> SNASIFKDLEALSFQSNASRNQDVFPILDLQELVICLQSCDFALATQENISRPTSDYMVTLYKQIIENFMGISVESLLNSSNQETGDGHLQEENENIYLDTLNVLVLNKICFKFFENIGVQDFNMTDLYKPEAQRTQRLLSAVVNYARFREERMFDCNS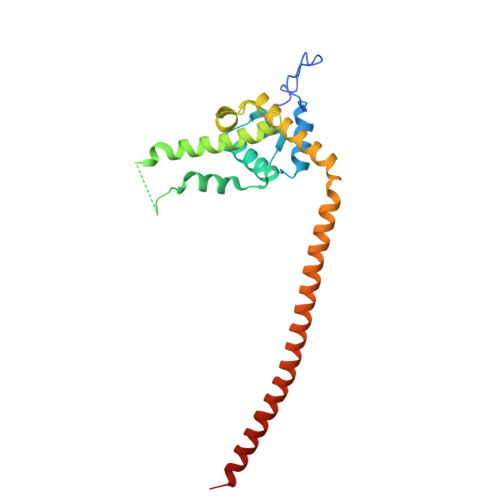FILQMESLLGQINKLNDEIKQLQKDFEVEVKEIEIEYSLLSGHINKYMNEMLEYMQ> GAGCAGACGTG;> ACTCCACTCA;> CAAGT;> T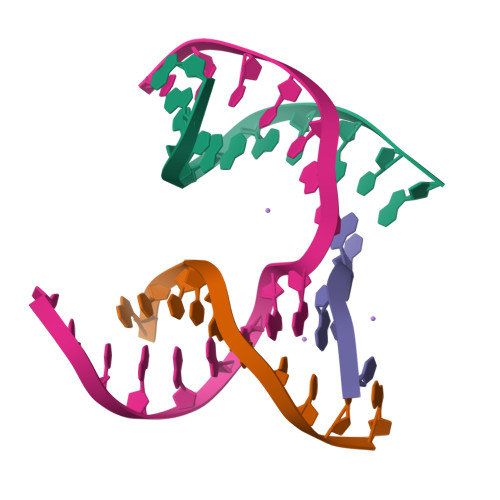CTGAGTGGCGTCTGC>MDIISVALKRHSTKAFDASKKLTPEQAEQIKTLLQYSPSSTNSQPWHFIVASTEEGKARVAKSAAGNYVFNERKMLDASHVVVFCAKTAMDDVWLKLVVDQEDADGRFATPEAKAANDKGRKFFADMHRKDLHDDAEWMAKQVYLNVGNFLLGVAALGLDAVPIEGFDAAILDAEFGLKEKGYTSLVVVPVGHHSVEDFNAT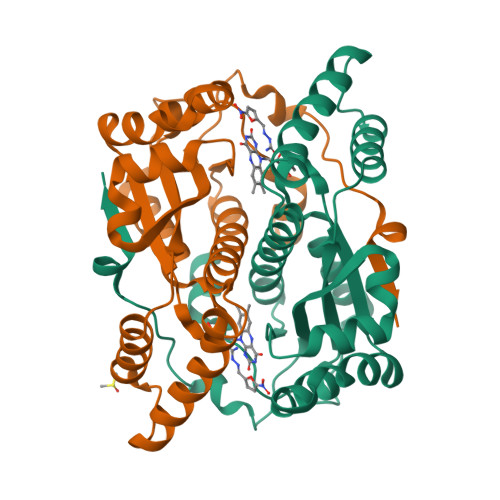LPKSRLPQNITLTEV[4x]>MSL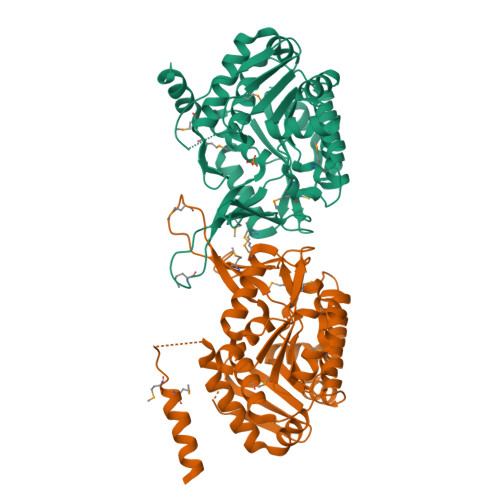KKTILCFGEALIDMLAQPLVKKGMPRAFLQCAGGAPANVAVAVARLGGAVQFVGMLGSDMFGDFLFDSFAEAGVVTDGIVRTSTAKTALAFVALDAHGERSFSFYRPPAADLLFRVEHFQDASFSDALIFHACSNSMTDADIAEVTFEGMRRAQAAGAIVSFDLNFRPMLWPNGENPASRLWKGLSLADVVKLSSEELDYLANTLAADANAVIQQLWQGRAQLLLVTDAAGPVHWYTRTAGGEVPTFRVQVQDSNAAGDAFVGGMLYTFAQQFDDAAALIDFCHDPESIVSTLRFAAAVGALAVTRQGAFTAMPMLSEVLSLIQEQSEGHHHHHH[2x]> MLPLTLLNATQGRPILVELKNGETFNGHLENCDNYMNLTLREVIRTMPDGDKFFRLPECYI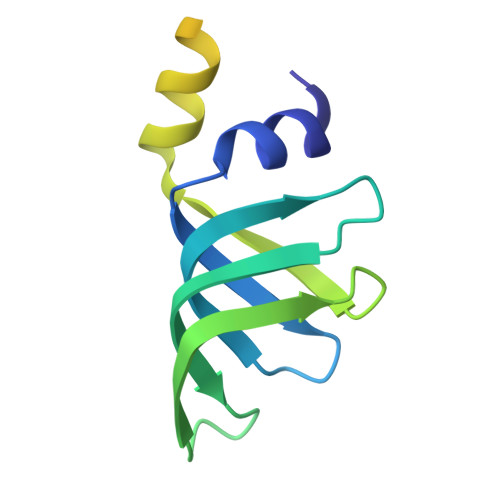RGNNIKYLRIQDEVLSQVAKQQAQQRENRGSRFRGRGQRGRGNYGHTAPNRRGRGRGGHMWSHPQFEK>YKKAGLQRTLVLIKPDAFERSLVAEIMGRIEKKNFKIVSMKFWSKAPRNLIEQHYKEHSEQSYFNDLCDFMVSGPIISIVYEGTDAISKIRRLQGNTNPLASAPGTIRGDLANDIRENLIHASDSEDSAVDEISIWFPE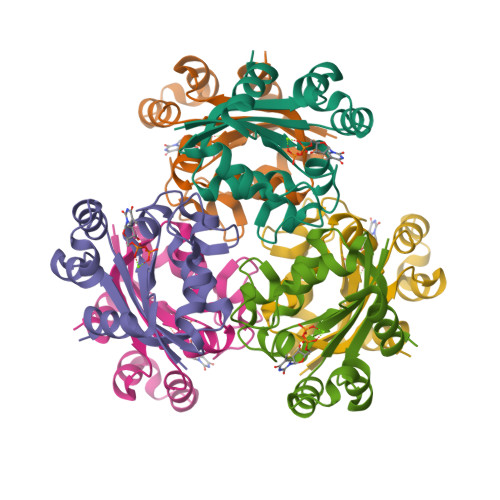TKMETDN[2x]> NLRQAVMLPEGEDLNEWIAVN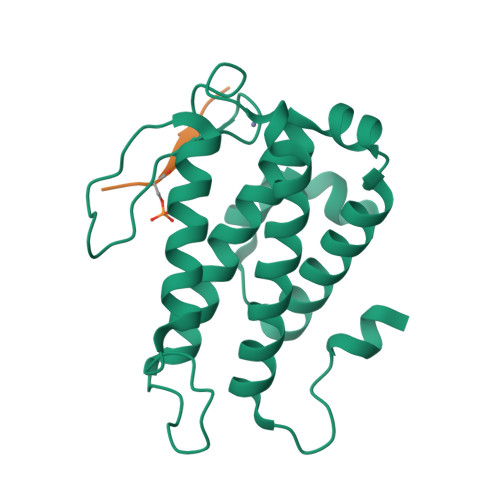TVDFFNQINMLYGTITEFCTEASCPVMSAGPRYEYHWADGTNIKKPIKCSAPKYIDYLMTWVQDQLDDETLFPSKIGVPFPKNFMSVAKTILKRLFRVYAHIYHQHFDSVMQLQEEAHLNTSFKHFIFFVQEFNLIDRRELAPLQELIEKL;> YHSVVRYA> IPTK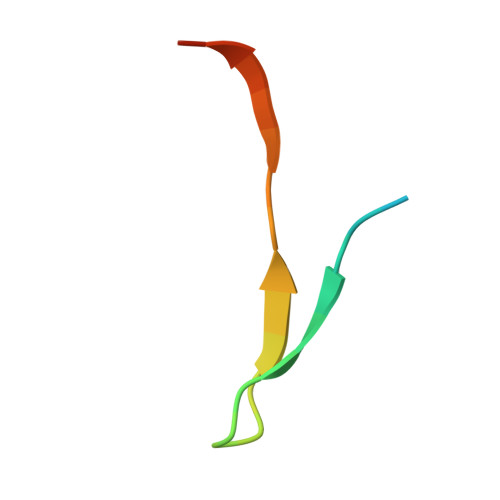FVQKVTITKEGKKRVAPQLLTTLSA N-DIMETHYL-LYSINE | C8 H18 N2 O2 | 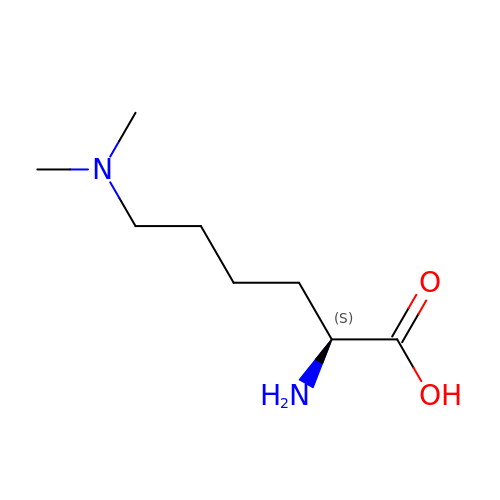XXEWFEBMSGLYBY-ZETCQYMHSA-N>MIQSQINRNIRLDLADAILLSKAKKDLSFAEIADGTGLAEAFVTAALLGQ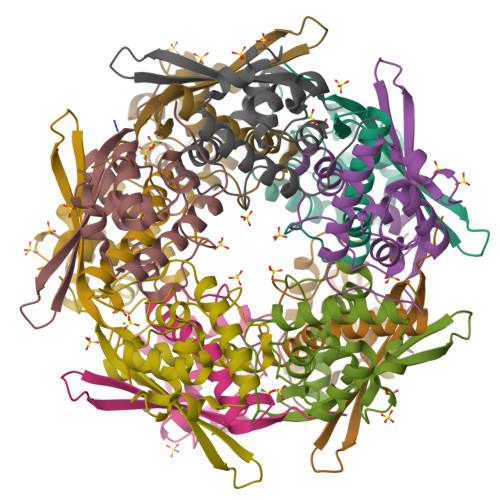QALPADAARLVGAKLDLDEDSILLLQMIPLRGCIDDRIPTDPTMYRFYEMLQVYGTTLKALVHEKFGDGIISAINFKLDVKKVADPEGGERAVITLDGKYGPTKPF[10x]(1R)-1-(4-chlorophenyl)ethyl carbamimidothioate 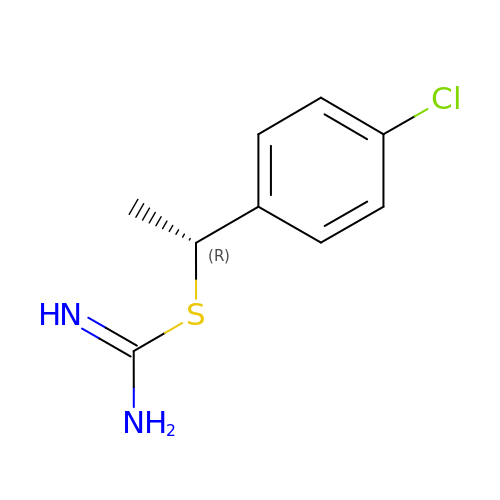| C9 H11 Cl N2 S | LMPMLIXDHLWEBJ-ZCFIWIBFSA-N>MHHHHHHGENLYFQGSMQPDMSLNVIKMKSSDFLESAELDSGGFGKVSLAFHRTQGLMIMKTVYKGPNCIEHNEALLEEAKMMNRLRHSRVVKLLGVIIEEGKYSLVMEYMEKGNLMHVLKAEMSTPLSVKGRIILEIIEGMAYLHGKGVIHKDLKPENILVDNDFHIKIADLGLASFKMWSKLNNEEHNELREVDGTAKKNGGTLYYMAPEHLNDVNAKPTEKSDVYSFAVVLWAIFANKEPYENAIAEQQLIMAIKSGNRPDVDDITEYCPREIISLMKLCWEANPEARP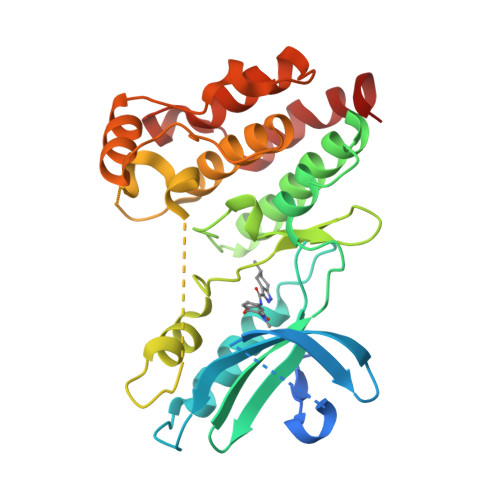TFPGIEEKFRPFYLSQLE[2x]> KFSPQLLSLLSLKTSLSGPPSAFQDWKVPVNGQNDAVWCSWSGVVCDNVTAQVISLDLSHRNLSGRIPIQIRYLSSLLYLNLSGNSLEGSFPTSIFDLTKLTTLDISRNSFDSSFPPGISKLKFLKVFNAFSNNFEGLLPSDVSRLRFLEELNFGGSYFEGEIPAAYGGLQRLKFIHLAGNVLGGKLPPRLGLLTELQHMEIGYNHFNGNIPSEFALLSNLKYFDVSNASLSGSLPQELGNLSNLETLFLFQNGFTGEIPESYSNLKSLKLLDFSSNQLSGSIPSGFSTLKNLTWLSLISNNLSGEVPEGIGELPELTTLFLWNNNFTGVLPHKLGSNGKLETMDVSNNSFTGTIPSSLCHGNKLYKLILFSNMFEGELPKSLTRCESLWRFRSQNNRLNGTIPIGFGSLRNLTFVDLSNNRFTDQIPADFATAPVLQYLNLSTNFFHRKLPENIWKAPNLQIFSASFSNLIGEIPNYVGCKSFYRIELQGNSLNGTIPWDIGHCEKLLSLNLSQNHLNGIIPWEISTLPSIADVDLSHNLLTGTIPSDFGSSKTITTFNVSYNQLIGPIPSGSFAHLNPSFFSSNEGLCGDLVGKPCN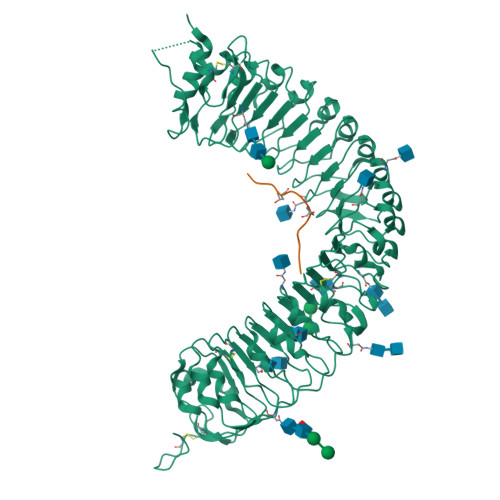SDSGLEVL;> HEVPSGPNPISN> MRSNKRQIIEKAIERKNEIETLPFDQNLAQLSKLNLKGETKTKYDAMKKDNVESTNKYLAPVEEKIHNAEALLDKFSFNASQSEIDDANELMDS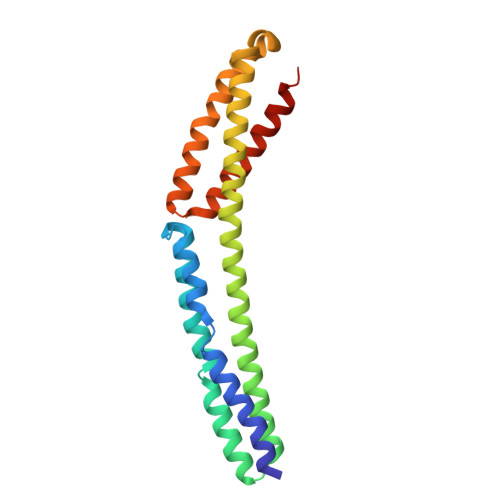YEQSYQQQLEDVNEIIALYKDNDELYDKCKVDYREMKRDVLANRHQFGEAASLLETEIEKFEPRLEQYEVLKADGNYVQAHNHIAALNEQMKQLRSYMHGSSGN>[4x]STGIAPKRYVYYPGSEELGPDEIRVIACGTGMPTARRAQAAAAWVVELGNGDKFIVDIGSGSMANIQSLMIPANYLTKIFLTHLHTDAWGDLVSMWAGGWTAGRTDPLEVWGPSGSREDMGTKYAVEHMLKAYNWDYMTRAVTINPRPGDINVHEFDYRA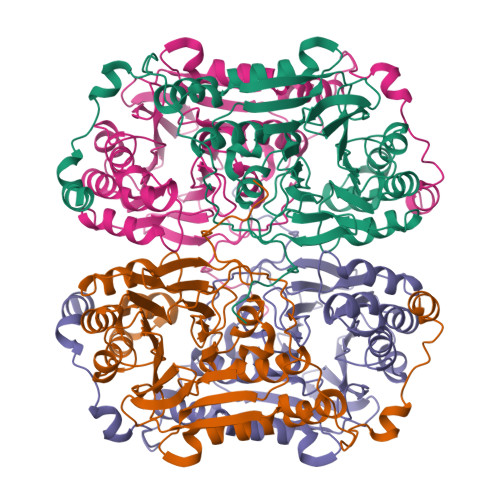LNEVVYQENGVTFRSWPCIHAGDGPVSFALEWNGYKVVFGGDTAPNIWYPEYAKGADLAIHECWMTSDQMMTKYNQPAQLALRINLDFHTSAQSFGQIMNMVQPRHAVAYHFFNDDDTRYDIYTGVRENYAGPLSMATDMMVWNITRDAVTERMAVSPDHAWDVAGPSEDLAPDRNRASEYTQYILDGRLNVDEANAHWKQEFMG>[2x]SAVLHPDSIYGTPLAPSWIKVKEKLVEATTAQRYLNRTEVEKICNDSGITDPGERKTLLGYLNNLGIVLYFEALDLSEIYVLDPHWVTIGVYRIINSSKTKNGHLNTSALGYILNEEQIRCDEYDPAKNNKFTYTLLEQRYLLDIMKQFELCYDEGKGLFIIPSNLPTQIDNEPEITEGEPLRFIMKYD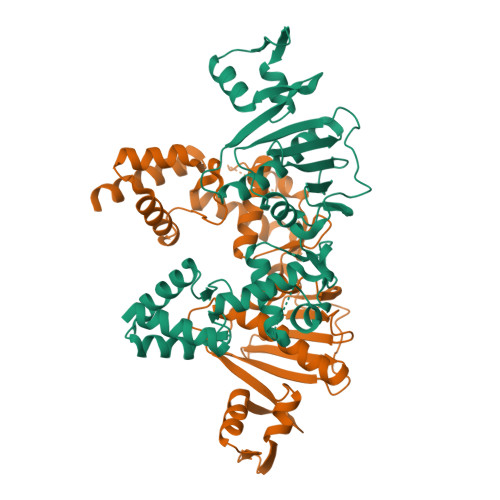YLPSTIIPRLMIAMQHQILDRMQWRYGMVLKSQDHEGALAKVVAETKDSTITIAIQGEPRCKREYLSIIWYEIKKINANFTNLDVKEFIPLPGHPDELVEYKELLGLEKMGRDEYVSGKLEKVFSVSKMLDSVISKEERNKER> KDTGATHDLVYHSKINTFVWDVEFDIVLSDSKELNKCYFVKCFNPYRINGKCDFAVSSIDIFSEGKRLLIENEFNFKITKAVHVATSKDVTEIVLHLSERISSPF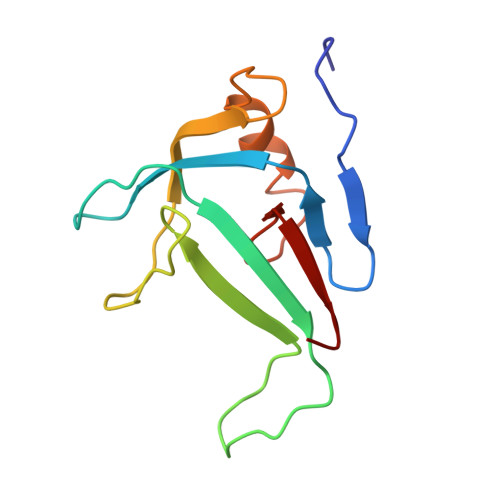PIVKEVVYLD> GPEGSQACAKGCELCSEV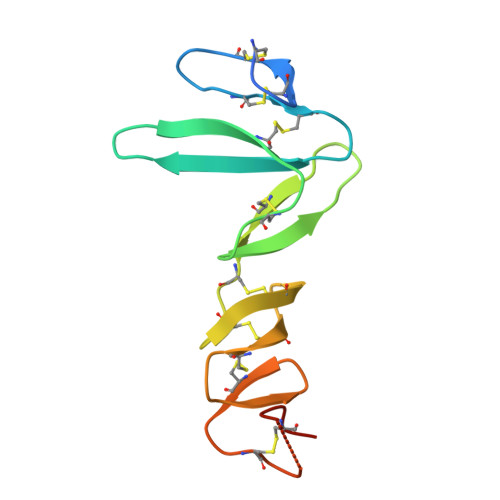NGCLKCSPKLFILLERNDIRQVGVCLPSCPPGYFDARNPDMNKCIKCKIEHCEACFSHNFCTKCKEGLYLHKGRCYPACPEGSSAANGTMECSSAAA>[3x]MPKYERTYTTQANFILHGGDYNPDQWLDRPDILQADLELMKLSHTNTFTVGVFAWSALEPEEGVYRFEWLDKVFDDIYRIGGRVILATPSGARPAWLSQKYPEVLRVNAARVRQLHGGRHNHCFTSSVYREKTQHINRLLAERYGDHPALLMWHVSNEYGGECHCNLCQEAFREWLKKKYNHDLDALNAAWWTSFWSHTYTDWSQIESPSPIGEHTIHGLNLDWKRFVTDQTISFFENEIVPLRELTPHIPITTNFMADTHDLIPFQGLDYSKFAKHLDVISWDAYPAWHNDWESTADLAMKVGFINDLYRSLKQQPFLLMACTPSLVNWHKVNKAKRPGMHFLSSMQMIAHGSDSILYFQWRKSRGSFEKFHGAVVDHDNRTDSRVFQEVAEVGKALKKMSGIVGTNRPAEVAILYDWE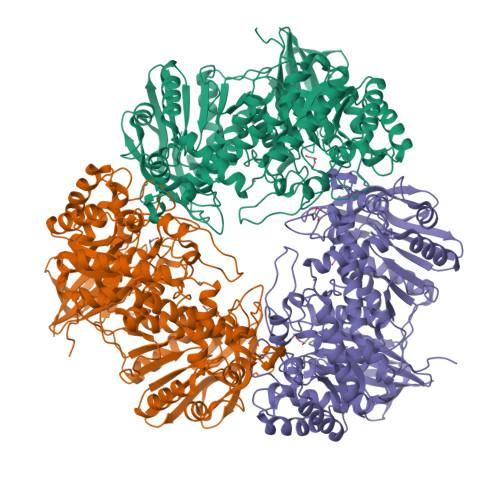NNWALNDAQGFAAETKRYPQTLVQHYRPFWERDIPVDVITKEHDFSRYKLLIAPMLYLVSEETIARLKEFVANGGTLVMTYISGIVDEHDLAYLGGWHQDLREMFGMEPIETDTLYPRDRNSVHYRGRSYELKDYATVIKIHAATVEGVYEDDFYADTPAVTSNQYGKGQAYYIGGRLEDQFHRDFYQELMEKLDLRPVLFVKHEKGVSVQARQAPECDYVFIMNFTEEKQAVVLEEKVKDLFTGEEIVGEIMLDKYEVRVVEKRR> MVDAVVTVFLEKTLNILEEKGRTVSDYRKQLEDLQSELKYMQSFLKDAERQKRTNETLRTLVADLRELVYEAEDILVDCQLADGDDGNEQRSSNAWLSRLHPARVPLQYKKSKRLQEINERITKIKSQVEPYFEFITPSNVGRDNGTDRWSSPVYDHTQVVGLEGDKRKIKEWLFRSNDSQLLIMAFVGMGGLGKTTIAQEVFNDKEIEHRFERRIWVSVSQTFTEEQIMRSILRNLGDASVGDDIGTLLRKIQQYLLGKRYLIVMDDVWDKNLSWWDKIYQGLPRGQGGSVIVTTRSESVAKRVQARDDKTHRPELLSPDNSWLLFCNVAFAANDGTCERPELEDVGKEIVTKCKGLPLTIKAVGGLLLCKDHVYHEWRRIAEHFQDELRGNTSETDNVMSSLQLSYDELPSHLKSCILTLSLYPEDCVIPKQQLVHGWIGEGFVMWRNGRSATESGEDCFSGLTNRCLIEVVDKTYSGTIITCKIHDMVRDLVIDIAKKDSFSNPEGLNCRHLGISGNFDEKQIKVNHKLRGVVSTTKTGEVNKLNSDLAKKFTDCKYLRVLDISKSIFDAPLSEILDEIASLQHLACLSLSNTHPLIQFPRSMEDLHNLQILDASYCQNLKQLQPCIVLFKKLLVLDMTNCGSLECFPKGIGSLVKLEVLLGFKPARSNNGCKLSEVKNLTNLRKLGLSLTRGDQIEEEELDSLINLSKLMSISINCYDSYGDDLITKIDALTPPHQLHELSLQFYPGKSSPSWLSPHKLPMLRYMSICSGNL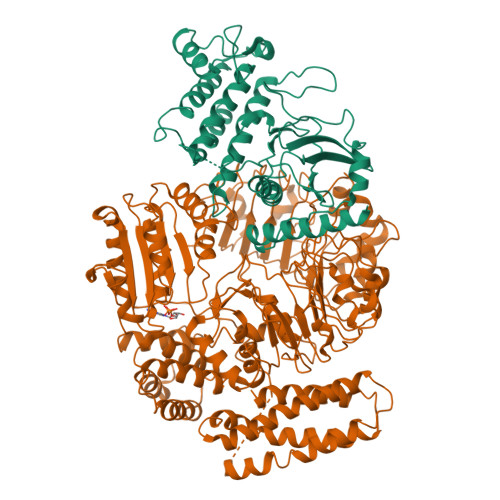VKMQEPFWGNENTHWRIEGLMLSSLSDLDMDWEVLQQSMPYLRTVTANWCPELESFAIEDVGFRGGVWMKTPLHRT;> MKKQYLKSGSGTRKEKDKAKRWFLDNGSIFLRELVADCNGKSIPIRSFSPEQILKATNNFDSSCFVSQDVYYKWYRGEIEDRSYMIKRFSEDEITGKRHRVKEVYNDIVLSARMSNHSNFLQLLGCCLEFPFPVLVFEFAEHGAMNQRGGVIVNGEESLLPWSVRLKIGKEIANAVTYLHTAFPKIIIHRDVKPMHVFLDKNWTAKLSDLSFSISLPEGKSRIEAEWVLGTFGYIDPLYHKTCFVTEYTDVYSFGICLLVIITGKPAIMTISDGDLQGILSLVRELCENGKLDEVIDPRLMKDITSGQRLQVEACVVLALRCCKERDEDRPKMIQVAKELKQIEASLKNSS>MRVPEKYSTLPAEDRSVHIVNICAIEDLGYLPSEGTLLNSLSVDPDAECKYGLYFRDGKRKVDYILVYHHKRASGSRTLARRGLQNDMVLGTRSVRQDQPLPGKGSPVDAGSPEVPMDYHEDDKRFRREEYEGNLLEAGLELENDEDTKIHGVGFVKIHAPWHVLCREAEFLKLKMPTKKVYHISETRGLLKTINSVLQKITDPIQPKVAEHRPQTTKRLSYPFSREKQHLFDLTDRDSFFDSKTRSTIVYEILKRTTCTKAKYSMGITSLLANGVYSAAYPLHDGDYEGDNVEFNDRKLLYEEWASYGVFYKYQPIDLVRKYFGEKVGLYFAWLGAYTQMLIPASIVGVIVFLYGCATVDENIPSMEMCDQRYNITMCPLCDKTCSYWKMSSACATARASHLFDNPATVFFSVFMALWAATFMEHWKRKQMRLNYRWDLTGFEEEEEAVKDHPRAEYEARVLEKSLRKESRNKETDKVKLTWRDRFPAYFTNLVSIIFMIAVTFAIVLGVIIYRISTAAALAMNSSPSVRSNIRVTVTATAVIINLVVIILLDEVYGCIARWLTKIEVPKTEKSFEERLTFKAFLLKFVNSYTPIFYVAFFKGRFVGRPGDYVYIFRSFRMEECAPGGCLMELCIQLSIIMLGKQLIQNNLFEIGIPKMKKFIRYLKLRRQSPSDREEYVKRKQRYEVDFNLEPFAGLTPEYMEMIIQFGFVTLFVASFPLAPLFALLNNIIEIRLDAKKFVTELRRPVAIRAKDIGIWY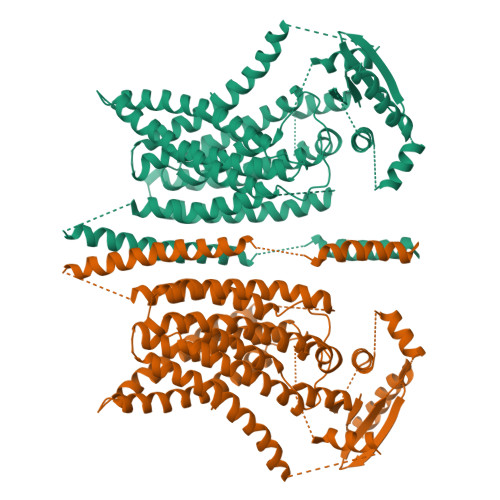NILRGVGKLAVIINAFVISFTSDFIPRLVYLYMYSQNGTMHGFVNHTLSSFNVSDFQNGTAPNDPLDLGYEVQICRYKDYREPPWSEHKYDISKDFWAVLAARLAFVIVFQNLVMFMSDFVDWVIPDIPKDISQQIHKEKVLMVELFMREEQGKQQLLDTWMEKEKPRDVPCNNHSPTTHPEAGDGSPVPSYEYHGDAL[2x]> MHFNTLTCVLVGLVAHTSAVPTKREAVNSCLTQAKVPTDAQGSQSWKEDGTAYNLRLPFEPAAIAVPTTVAQVSAAVECGAKHGVAISAKSGGHSYTSLGFGGEDGHLMIELDRMYSVKLAKDGTAKIQPGARLGHVATELWNQGKRALAHGTCPGVGLGGHALHGGYGMVARKHGLTLDLMIGATVVLPTGKVVHCSKTENSDLFWGIRGAGANFGVVVELEFQTFAAPEKITYFDIGLNWDQNTAPQGLYDFQEFGKGMPAEITMQMGVSKNGYSVDGAYIGDEASLRKALQPLVQKFGGVQVTATTVDWMGLVTHFAGAGVNVNPTSASYDAHDNFYASSLAAPALTLAEFKSF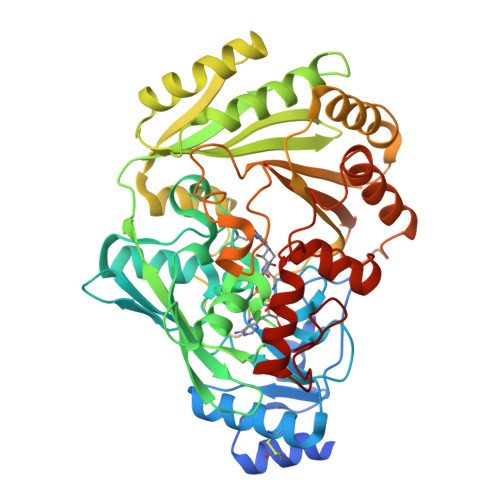VNFVSTTGKSSSHSWWLQMDITGGTYSAVSKPKPSDTAYVHRDTLLLFQFYDSVAATAQYPSDGFNLIKGLRQSISSSLKAGTWGMYANYPDSQIKNDRATEMYWGSNVAKLEAVKAKYDPKNLFRNPQSIKPKA> N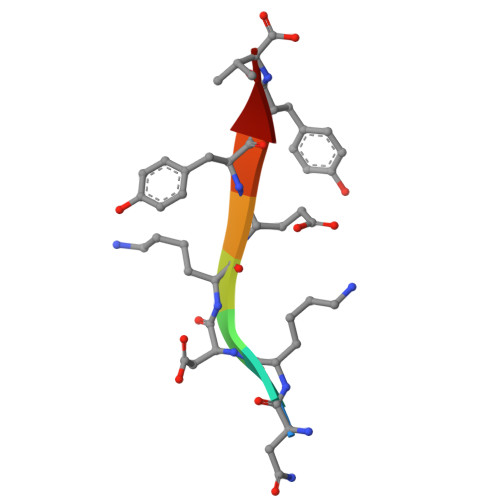KDKEYYV However, intestinal bacterial GUSs cleave the attached glucuronic acid for use as a carbon source, allowing potentially toxic compounds to re-enter the enterohepatic circulation. However, microflora-encoding β-glucuronidases (GUSs) are notorious for reversing the glucuronidation to release SN-38 in the intestinal lumen and thus represent the major cause of undesirable effects. GUS contains a deep enzyme active site (the two catalytic glutamates lie ~12 Å below the protein surface). To understand the underlying structural basis, we prepared C6-propyl, -hexyl, and -nonyl UIFGs (2–4, respectively) and resolved the eight X-ray crystal structures of 1–4 bound to EcGUS or Bifidobacterium dentium GUS (BdGUS).

Because the resolutions of the four structures for BdGUS (1.7–2.4 Å) were higher than those for EcGUS (2.5–3.2 Å), water molecules could be visualized in the catalytic site. Water molecules I–III were conserved in all of the BdGUS structures and located near the UIFG-binding moiety to mediate interactions between the inhibitor and certain residues. Interestingly, waters V–VII were absent in the inhibitors 3- and 4-bound forms. The alkyl substituents of 2–4 appear to expel some of the water molecules. f Superimposition of inhibitors 1–4 in the crystal structures. However, LgGUS and BdGUS have more spacious aglycone-binding sites than EcGUS and CpGUS, explaining why 2–4 did not have high affinity for LgGUS and BdGUS. To develop inhibitors with higher affinity for LgGUS and BdGUS, a bulkier group should be considered, e.g., phenyl group.

>NGMLYPQSNDSRIVFPLDGVWDFRTAGEDSYPAEWADAPLPEPLPMAVPGSYNDQNDELNLRAHYGWVVYQRSFAVPSRLVAGQRMILRFDAATHAADVYLNGQLLGSHFGGFLPFEFDVTSALHAGENLLTVAVDNRIGSSTLPVGNDAGTAFMGSDNANVPAVAEAKKHARRQNLPNFDFFNFAGLNRHVELYTTPADAYIADIAITTERLDHIAGDACTAANALIAYDVTFGGDFPSNPTDPNTPIQPSDPAINHADSSESAESDIQRATTYGRQVRISILDGEGTVVAGVTADIERSGDGTAKASGEIAIRDAKLWNPGAAYLYTAVAELLPEGGAESSSRIIDAYRQTFGIRTVEVSGTTFLINGKPFYFKGFGKHEDSYFHGRGTDDVLNVKDVSLIHWLHANSFRTSHYPYAESMYDLCDREGIVIIDEVPAVGMSWLQYANPLVAERHREAIRGMIARDKNHPCIVMWSIANEPGLDGDGERPRQAYDYFRPLYELAHASDPQNRPVTLVCCQNDYTTDITERTMDVVCINRYYGWYNLSGDLDAACHALNIELDFWENIGKPVMFTEYGADTIEGIHGTHGEMFSEEFQRDYYARINAEIDKRPWFIGEQLWNFADFATFQGIIRVEGNRKGILTRDRQPKMAAHWLRERWAGIPDYGYKG[4x]>SMKITSSNFATIATSENFAKLSVLPKNHREPIK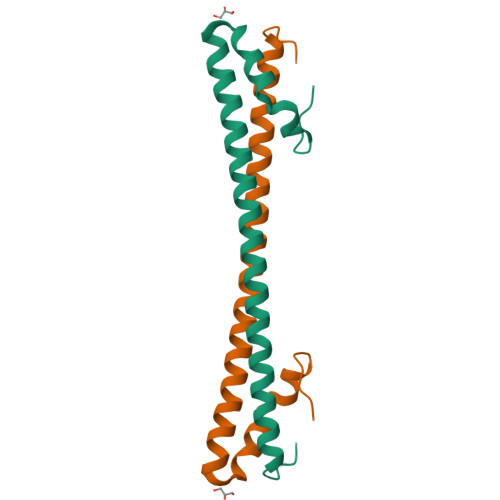GLFKSAVEQFSSARDFFKNENYSKELAEKFNKEAVNEAVEKLQKAIDLAEKQGIQF[2x]Within this complex, UvrA acts as the initial damage sensor but hands off the lesion-containing DNA to UvrB and dissociates, leaving UvrB bound to the lesion in a preincision complex, the precise nature of which is not known. Both UvrA and UvrB expend ATP to form the preincision complex, which is believed to require threading of a β-hairpin element on UvrB through the DNA duplex. UvrB presents the lesion-containing strand to UvrC, which catalyzes hydrolysis of the 5th phosphodiester bond 3′ to the lesion and then the 8th phosphodiester bond 5′ to the lesion. UvrB is classified as a member of SF2 helicases on the basis of conserved helicase motifs (I-VI) (Supplementary ).

If the UvrB helicase domain underwent rigid-body movements similar to those seen for other helicases as proposed previously, ATP-dependent domain closure would force the F-loop toward DNA, perhaps causing F527 to intercalate into the duplex stack, which may function as a “ratchet” to facilitate unidirectional translocation upon ATP-hydrolysis. Indeed, in a structure we determined of UvrB (S91C) bound to a fully base-paired DNA duplex, F527 is intercalated into a sharply bent DNA duplex; furthermore, the crystal structure of the analogous complex containing a F527A mutation revealed substantially reduced DNA bending (Supplementary ) and increased DNA disorder presumably due to the loss of “ratchet” that seems to lock the duplex DNA in position. That F527 intercalation is important functionally suggested by the reduced incision efficiency observed for the F527A mutant UvrB.

> VEGRFQLVAPYEPQGDQPQAIAKLVDGLRRGVKHQTLLGATGTGKTFTISNVIAQVNKPTLVIAHNKTLAGQLYSELKEFFPHNAVEYFVCYYDYYQPEAYVPQTDTYIEKDAKINDEIDKLRHSATSALFERRDVIIVASVSSIYGLGSPEEYRELVVSLRVGMEIERNALLRRLVDIQYDRNDIDFRRGTFRVRGDVVEIFPASRDEHSIRVEFFGDEIERIREVDALTGEVLGEREHVAIFPASHFVTREEKMRLAIQNIEQELEERLAELRAQGKLLEAQRLEQRTRYDLEMMREMGFSSGIENYSRHLALRPPGSTPYTLLDYFPDDFLIIVDESHVTLPQLRGMYNGDRARKQVLVDHGFRLPSALDNRPLTFEEFEQKINQIIYVSATPGPYELEHSPGVVEQIIRPTGLLDPTIDVRPTKGQIDDLIGEIRERVERNERTLVTTLTKKMAEDLTDYLKEAGIKVAYLHSEIKTLERIEIIRDLRLGKYDVLVGINLLREGLDIPEVSLVAILDADKEGALRSERSLIQTIGRAARNANGHVIMYADTITKSMEIAIQETKRRRAIQEEYNRKHGIVPRTVKKEIR> MDNNYHFWGNGDRQDVSLSYEDYYSILDCLLDEKLSPQGLMKFKNLHEVSMYGVSYVPLYCFPVAYGISHMLTGKVRRGHSGYRNLFSLMSVVLPFTCWYAYT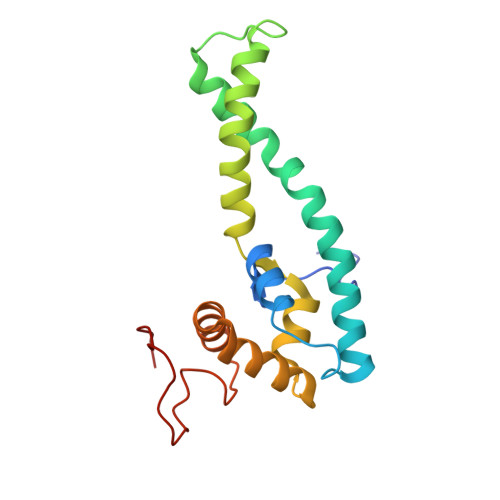TPIPRRLYTEIICSNNADGAYVRNRIKQQKPGIWRKLSQQLYNKNFRFPELNQDLTATEFPLDYVAPHKF> MDYKDDDDKLAEHGESSEDRISEIDYEFLPELSALLGVDAFQVAKSQEEEEHKERMKMKKGFNSQMRSEAKRLKTFETYDTFRSWTPQEMAAAGFYHTGVRLGVQCFCCSLILFGNSLRKLPIERHKKLRPECEFLQGKDVGNIGKYDIRVKRPEKMLRGGKARYHEEEARLESFEDWPFYAHGTSPRVLSAAGFVFTGKRDTVQCFSCGGSLGNWEEGDDPWKEHAKWFPKCEFLQSKKSSEEIAQYIQSYEGFVHVTGEHFVKSWVRRELPMVSAYCNDSVFANEELRMDMFKDWPQESPVGVEALVRAGFFYTGKKDIVRCFSCGGCLEKWAEGDDPMEDHIKFFPECVFLQTLKSSAEVIPTLQSQYALPEATETTRESNHGDAAAVHSTVVDLGRSEAQWFQEARSLSEQLRDNYTKATFRHMNLPEVCSSLGTDHLLSCDVSIISKHISQPVQEALTIPEVFSNLNSVMCVEGETGSGKTTFLKRIAFLWASGCCPLLYRFQLVFYLSLSSITPDQGLANIICAQLLGAGGCISEVCLSSSIQQLQHQVLFLLDDYSGLASLPQALHTLITKNYLSRTCLLIAVHTNRVRDIRLYLGTSLEIQEFPFYNTVSVLRKFFSHDIICVEKLIIYFIDNKDLQGVYKTPLFVAAVCTDWIQNASAQDKFQDVTLFQSYMQYLSLKYKATAEPLQATVSSCGQLALTGLFSSCFEFNSDDLAEAGVDEDEKLTTLLMSKFTAQRLRPVYRFLGPLFQEFLAAVRLTELLSSDRQEDQDLGLYYLRQIDSPLKAINSFNIFLYYVSSHSSSKAAPTVVSHLLQLVDEKESLENMSENEDYMKLHPQTFLWFQFVRGLWLVSPESSSSFVSEHLLRLALIFAYESNTVAECSPFILQFLRGKTLALRVLNLQYFRDHPESLLLLRSLKVSINGNKMSSYVDYSFKTYFENLQPPAIDEEYTSAFEHISEWRRNFAQDEEIIKNYENIRPRALPDISEGYWKLSPKPCKIPKLEVQVNNTDAADQALLQVLMEVFSASQSIEFRLFNSSGFLESICPALELSKASVTKCSMSRLELSRAEQELLLTLPALQSLEVSETNQLPEQLFHNLHKFLGLKELCVRLDGKPNVLSVLPREFPNLLHMEKLSIQTSTESDLSKLVKFIQNFPNLHVFHLKCDFLSNCESLMAVLASCKKLREIEFSGRCFEAMTFVNILPNFVSLKILNLKDQQFPDKETSEKFAQALGSLRNLEELLVPTGDGIHQVAKLIVRQCLQLPCLRVLTFHDILDDDSVIEIARAATSGGFQKLENLDISMNHKITEEGYRNFFQALDNLPNLQELNICRNIPGRIQVQATTVKALGQCVSRLPSLIRLHMLSWLLDEEDMKVINDVKERHPQSKRLIIFWKLIVPFSPVILE;> MHHHHHHMAQV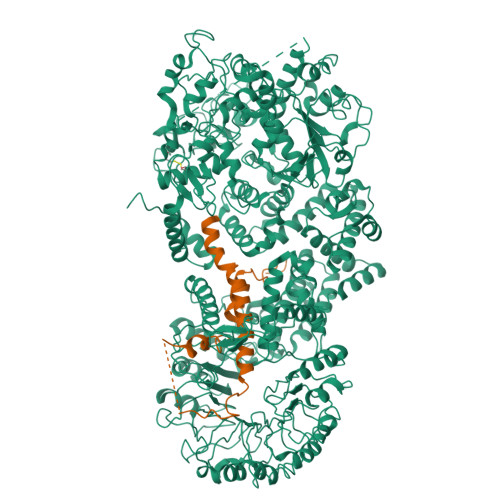INTNSLSLLTQNNLNKSQSALGTAIERLSSGLRINSAKDDAAGQAIANRFTANIKGLTQASRNANDGISIAQTTEGALNEINNNLQRVRELAVQSANSTNSQSDLDSIQAEITQRLNEIDRVSGQTQFNGVKVLAQDNTLTIQVGANDGETIDIDLKQINSQTLGLDTLNVQQKYKVSDTAATVTGYADTTIALDNSTFKASATGLGGTDQKIDGDLKFDDTTGKYYAKVTVTGGTGKDGYYEVSVDKTNGEVTLAGGATSPLTGGLPATATEDVKNVQVANADLTEAKAALTAAGVTGTASVVKMSYTDNNGKTIDGGLAVKVGDDYYSATQNKDGSISINTTKYTADDGTSKTALNKLGGADGKTEVVSIGGKTYAASKAEGHNFKAQPDLAEAAATTTENPLQKIDAALAQVDTLRSDLGAVQNRFNSAITNLGNTVNNLTSARSRIEDSDYATEVSNMSRAQILQQAGTSVLAQANQVPQNVLSLLR Enolase is a glycolytic enzyme that requires a divalent metal ion (optimally Mg2+) bound in the active site to catalyze the dehydration of 2-phosphoglycerate (2-PG) to phosphoenolpyruvate (PEP), as well as the reverse reaction in the gluconeogenesis pathway. Interestingly, enolase has been identified on the cell surface of S. aureus, enhancing the staphylokinase activation of plasminogen. The Sa_enolase monomer has two distinct domains, a small N-terminal domain (residues 1–137) and a large C-terminal barrel domain (residues 149–434), connected by a linker region (residues 138–148). Biochemical and structural studies indicate that the octameric form of Sa_enolase is enzymatically active in vitro and likely also in vivo, while the dimeric form is catalytically inactive and may be involved in other biological processes.

Moreover, the structure of Sa_enolase in complex with PEP was also determined at 1.6 Å resolution, enabling the elucidation of the interaction network between the enzyme and PEP. PEP-bound Sa_enolase crystals were obtained by the co-crystallization of Sa_enolase with the substrate 2-PG. The crystals belonged to space group I4, with two monomers forming a single homodimer in the asymmetric unit. Interestingly, L1 in the PEP-bound structure of Sa_enolase displays both the ‘open’ and ‘closed’ conformations. Lys343, Lys394, Asp318, Arg372 and Ser373, together with Ser42 from L1, constitute this inter­action network. On the opposite side, the PEP phosphate group forms hydrogen bonds to Arg372, Ser373 and Ser42. Although enolase is a metalloenzyme containing two metal-binding sites in the active site, our structure only displays one bound Mg2+ ion near the PEP carboxyl group. As shown in Fig. 3(d), two PEP carboxyl O atoms occupy two positions within the Mg2+-binding site through coordinate bonds. To the best of our knowledge, the structure of the PEP-bound form of Sa_enolase constitutes the first Gram-positive bacterial structure solved with ligand bound and displaying evidence of catalytic loop shifting within the active site.

>MPIITDVYAREVLDSRGNPTVEVEVLTESGAFGRALVPSGASTGEHEAVELRDGDKSRYLGKGVTKAVENVNEIIAPEIIEGEFSVLDQVSIDKMMIALDGTPNKGKLGANAILGVSIAVARAAADLLGQPLYKYLGGFNGKQLPVPMMNIVNGGSHSDAPIAFQEFMILPVGATTFKESLRWGTEIFHNLKSILSKRGLETAVGDEGGFAPKFEGTEDAVETIIQAIEAAGYKPGEEVFLGFDCASSEFYENGVYDYSKFEGEHGAKRTAAEQVDYLEQLVDKYPIITIEDGMDENDWDGWKQLTERIGDRVQLVGDDLFVTNTEILAKGIENGIGNSILIKVNQIGTLTETFDAIEMAQKAGYTAVVSHRSGETEDTTIADIAVATNAGQIKTGSLSRTDRIAKYNQLLRIEDELFETAKYDGIKSFYNLDKLEHHHHHH[2x]>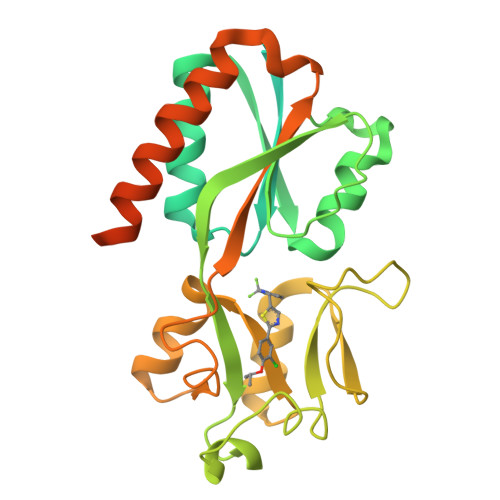[2x]MPIHNLNHVNMFLQVIASGSISSAARILRKSHTAVSSAVSNLEIDLCVELVRRDGYKVEPTEQALRLIPYMRSLLNYQQLIGDIAFNLNKGPRNLRVLLDTAIPPSFCDTVSSVLLDDFNMVSLIRTSPADSLATIKQDNAEIDIAITIDEELKISRFNQCVLGYTKAFVVAHPQHPLCNASLHSIASLANYRQISLGSRSGQHSNLLRPVSDKVLFVENFDDMLRLVEAGVGWGIAPHYFVEERLRNGTLAVLSELYEPGGIDTKVYCYYNTALESERSFLRFLESARQRLRELGRQRFDDAPAWQPSIVETAQRRSGPKALAYRQRAAPE>[2x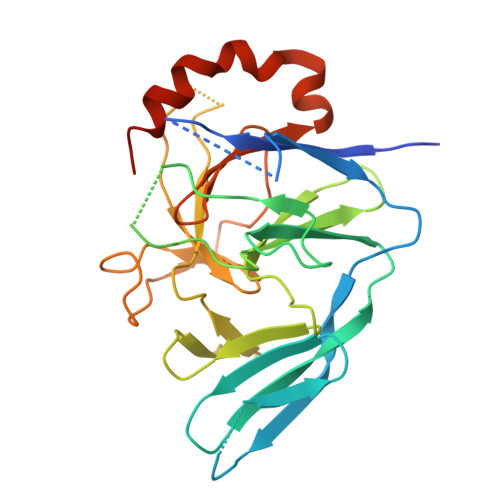]GSEEHCAPNKEPVKYGELVVLGYNGALPNGDRGRRKSRFALYKRPKANGVKPSTVHVISTPQASKAISCKGQHSISYTLSRNQTVVVEYTHDKDTDMFQVGRSTESPIDFVVTDTISGSQNTDEAQITQSTISRFACRIVCDRNEPYTARIFAAGFDSSKNIFLGEKAAKWKNPDGHMDGLTTNGVLVMHPRGGFTEESQPGVWREISVCGDVYTLRETRSAQQRGKLVESETNVLQDGSLIDLCGATLLWRTADGLFHTPTQKHIEALRQEINAARPQCPVGLN> MEVNEKAPAQARPTVFRWT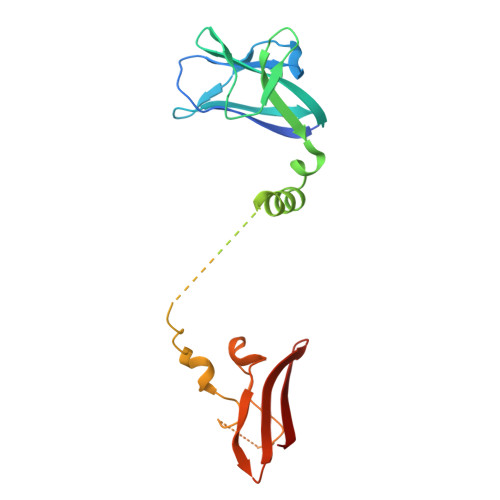GGGKEVYLSGSFNNWSKLPLTRDHNNFVAILDLPEGEHQYKFFVDGQWTHDPSEPIVTSQLGTVNNIIQVKKTDFEVFDALMVDSQKCSDVSELSSSPPGPYHQEPYISKPEERFKAPPILPPHLLQVILNKDTGISCDPALLPEPNHVMLNHLYALSIKDGVMVLSATHRYKKKYVTTLLYKPI LASV has a surface-displayed class-I trimeric glycoprotein spike complex that mediates receptor recognition and fusion of the viral and host-cell membranes at acidic pH. The spike complex consists of three copies of a single polypeptide chain that is cleaved twice to give a structured signal peptide, a receptor-binding module (GP1), and a trans-membrane module (GP2). We previously showed that a triad of histidines on GP1 is important for binding LAMP1, and we further demonstrated that the binding of LAMP1 triggers the spike of LASV to catalyze membrane fusion by potentiating its response to pH. We present a crystal structure of the GP1 domain from the Morogoro (MORV) OW mammarenavirus, which does not interact with LAMP1, and conduct a comparative structural analysis between GP1 of MORV and LASV (GP1MORV and GP1LASV, respectively) to identify structural differences related to the ability to bind LAMP1.

Similarly to GP1LCMV-Fc, GP1MORV-Fc did not pull down LAMP1 from HEK293T cells, nor did it interact with recombinant LAMP1 immobilized on a sensor chip. We obtained crystals of GP1MORV (residues 73 to 235) at pH 4.0. The asymmetric unit contained a total of 16 copies of GP1MORV, mostly differing in the extent of electron density observed for their N-linked glycans, which in some cases were stabilized by a nearby protein molecule. GP1MORV has a central β–sheet made of five β-strands, flanked by the domain termini on one side and helices and loops on the other. The global structure of GP1MORV is similar to the previously determined structure of GP1LASV. The histidine triad in GP1MORV (His91, His92, and His228 according to GPCMORV numbering) adopts the same conformation as the triad in GP1LASV. GPCMORV has a β-hairpin made of two β-strands (β5 & β6) stabilized by a disulfide bridge (D3) against α3. This β-hairpin is divergent in sequence and was previously termed the variable region of GP1LASV. GP1LASV has a strong positive charge in the vicinity of the triad, whereas this charge on the GP1MORV surface seems milder. Overall, the structure of GP1MORV does not reveal major global structural differences that could account to the inability to bind LAMP1.

>[16x]SHHHHHHGGMSGLNATMPLSCSKNNSHHYIQVRNDTGLELTLTNTSLLDHKFCNLSDAHKRNLYDKALMSIVTTFHLNIPNFNQYEVMSCDFNGGKITVQYNLSHSSYVDAANHCGTIANGIMDTFRRMYWSNALSPSEYISGTTCIQTAYQYLIIQNTTWEDHCVFSRPS(3E,5E,7E,9E,11E,13E)-pentadeca-3,5,7,9,11,13-hexaen-2-one 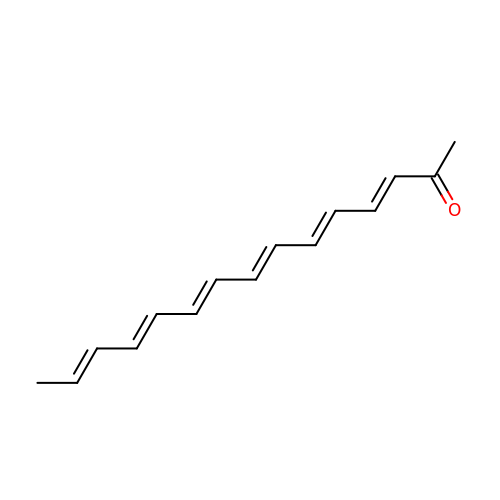| C15 H18 O | IKKRHADMXZRWGK-IDFWPVMJSA-N Isocitrate dehydrogenases (IDHs) are a family of enzymes responsible for the oxidative decarboxylation of isocitrate (ICT) into α-ketoglutarate (α-KG) using NAD or NADP as coenzyme with the concomitant production of NADH or NADPH. Mammalian NAD-IDHs are comprised of three types of subunits in the ratio of 2α:1β:1γ with similar molecular masses of 37 kDa, 39 kDa and 39 kDa, respectively. The α and β subunits form a heterodimer (αβ) and the α and γ subunits form another heterodimer (αγ), which are assembled into a heterotetramer (α2βγ) and further into a heterooctamer (the heterotetramer and heterooctamer are called the holoenzyme). In addition, our biochemical data showed that in the holoenzyme, both α subunits have catalytic activity; in contrast, the γ subunit plays a regulatory role, whereas the β subunit plays a structural role to facilitate the assembly of the holoenzyme.

However, we were able to grow crystals of the αγ heterodimer with the active site bound with Mg2+ and the allosteric site bound with Mg2+, CIT and ATP from a crystallization solution containing CIT and a relatively low concentration of ATP (2 mM). This led to the determination of the structure of the αMgγMg+CIT+ATP heterodimer. In the αMgγMg+CIT+ATP structure, there is ATP bound to the ADP binding site of the allosteric site, which stabilizes CIT binding through Mg2+-mediated interactions and leads the enzyme to adopt an active conformation. This provides the structural basis for why the enzyme can be activated by low concentrations of ATP. Structural analysis shows that ATP occupies the ADP binding site, and particularly the adenine and α-phosphate of ATP make very similar interactions with the surrounding residues as those of ADP. , the β- and γ-phosphates of ATP are oriented away from the Mg2+-binding site and make different interactions with the enzyme due to potential steric conflicts with the surrounding residues. Meanwhile, a water molecule occupies the position of the β-phosphate of ADP and mediates the interaction between the Mg2+ and the α-phosphate of ATP. As a result, the interaction between ATP and Mg2+ is mediated via a water molecule instead of the direct interaction between ADP and Mg2+, suggesting that the stabilization of the CIT and Mg2+ binding by ATP is weaker than the stabilization by ADP. Structural comparisons with the previously reported αγ structures show that the αMgγMg+CIT+ATP and αMg+ATPγMg+CIT+ATP structures are more similar to the active αMgγMg+CIT+ADP structure (RMSD of 0.26 Å and 0.56 Å for about 650 Cα atoms, respectively) than the inactive αMgγ structure (RMSD of 1.0 Å and 1.1 Å for about 650 Cα atoms, respectively). In the αMgγMg+CIT+ATP structure, there is Mg2+ bound at the active site, and in the αMg+ATPγMg+CIT+ATP structure, there are both Mg2+ and ATP bound at the active site.

> MGSTGGVQTVTLIPGDGIGPEISAAVMKIFDAAKAPIQWEERNVTAIQGPGGKWMIPSEAKESMDKNKMGLKGPLKTPIAAGHPSMNLLLRKTFDLYANVRPCVSIEGYKTPYTDVNIVTIRENTEGEYSGIEHVIVDGVVQSIKLITEGASKRIAEFAFEYARNNHRSNVTAVHKANIMRMSDGLFLQKCREVAESCKDIKFNEMYLDTVCLNMVQDPSQFDVLVMPNLYGDILSDLCAGLIGGLGVTPSGNIGANGVAIFESVHGTAPDIAGKDMANPTALLLSAVMMLRHMGLFDHAARIEAACFATIKDGKSLTKDLGGNAKCSDFTEEICRRVKDLD;> MGSFSEQTIPPSAKYGGRHTVTMIPGDGIGPELMLHVKSVFRHACVPVDFEEVHVSSNADEEDIRNAIMAIRRNRVALKGNIETNHNLPPSHKSRNNILRTSLDLYANVIHCKSLPGVVTRHKDIDILIVRENTEGEYSSLEHESVAGVVESLKIITKAKSLRIAEYAFKLAQESGRKKVTAVHKANIMKLGDGLFLQCCREVAARYPQITFENMIVDNTTMQLVSRPQQFDVMVMPNLYGNIVNNVCAGLVGGPGLVAGANYGHVYAVFETATRNTGKSIANKNIANPTATLLASCMMLDHLKLHSYATSIRKAVLASMDNENMHTPDIGGQGTTSEAIQDVIRHIRVINGRAVEA> MSTLGHQYDNSLVSNAFGFLRLPMNFQPYDSDADWVITGVPFDMATSGRAGGRHGPAAIRQVSTNLAWEHNRFPWNFDMRERLNVVDCGDLVYAFGDAREMSEKLQAHAEKLLAAGKRMLSFGGDHFVTLPLLRAHAKHFGKMALVHFDAHTDTYANGCEFDHGTMFYTAPKEGLIDPNHSVQIGIRTEFDKDNGFTVLDACQVNDRSVDDVIAQVKQIVGDMPVYLTFDIDCLDPAFAPGTGTPVIGGLTSDRAIKLVRGLKDLNIVGMDVVEVAPAYDQSEITALAAA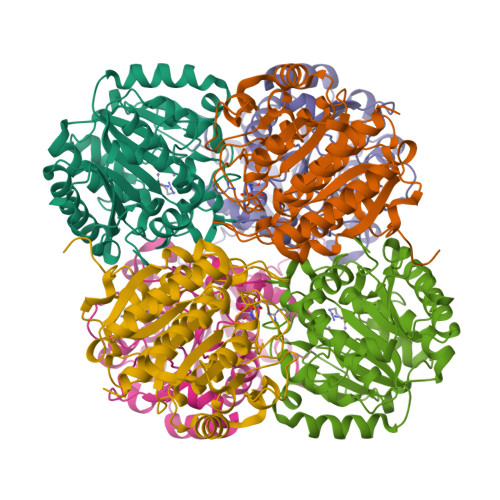TLALEMLYIQAAKKGE> MFEKLYSAIIYSDEFKKILLGRGVDDLEIASAYIAFLYEDLPIIGKNLCAAFLRMGL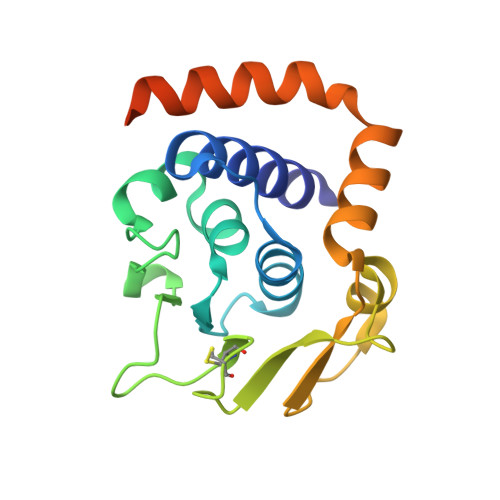DAVYNVMPSGKVYSPRHKLYPISRYGIDGVCINCDGGKIILRISNKGYDPEDLLESKGLESRIFVSKNFKKKSMEIIEKIWDVNKIRLIARKEILERISAGGILHMIRLEHHHHHH>[2x]AQKPVDNITQIIGGTPVVKLRNVVDDNAADVYVKLEYQNPGGSVKDRIA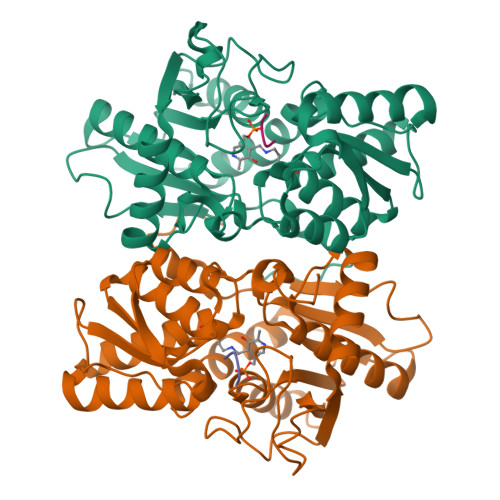LAMIEKAEREGKIKPGDTIVEPTSGNTGIGLAFVCAAKGYKAVFTMPETMSQERRNLLKAYGAELVLTPGSEAMKGAIKKAKELKEEHGYFEPQQFENPANPEVHELTTGPELLQQFEGKTIDAFLAGVGTGGTLSGVGKVLKKEYPNIEIVAIEPEASPVLSGGEPGPHKLQGLGAGFIPGTLNTEIYDSIIKVGNDTAMEMSRRVAKEEGILAGISSGAAIYAAIQKAKELGKGKTVVTVLPSNGERYLSTPLYS;>[2x]YMFYI RTX adhesins are long, multi-domain proteins present on the outer membrane of many Gram-negative bacteria. To expand the reach of the ligand-binding domains, RTX adhesins maintain a central extender region of multiple tandem repeats, which makes up most of the proteins’ large molecular weight. In this study, we analyzed extender regions from two additional RTX adhesins, including the long adhesion proteins from Marinobacter hydrocarbonoclasticus (MhLap) – an oil-eating marine bacterium – and Aeromonas hydrophila (AhLap) – an opportunistic pathogen of fish and mammals. However, all the tetra-tandemers have at least one calcium ion coordinated in the linker region between beta-sandwich domains whose role appears to be the rigidification of the extender region to help the adhesin extend its reach.

Calcium SAD phasing (Guo et al., 2019a, Guo et al., 2019b) was used to solve the tetra-tandemer structures to 2.0 Å (MhLap) and 1.75 Å resolution (AhLap). The repeats are rotated relative to each other around the long central axis, producing a handedness to the tetra-tandemers reminiscent of helices. Both the MhLap and AhLap structures show right-handed rotations, with pitches of approximately i + 3 and i + 2, respectively. Alternatively, the AhLap repeats possess a more involved connectivity, resulting in 50 Å-long beta sandwiches that are held together by one four-stranded and another five-stranded beta sheet. The AhLap tetra-tandemer coordinates many more calcium ions throughout its length than does MhLap, although the number of ions per repeat is inconsistent. Each inter-domain interface contains, at minimum, three highly coordinated Ca2+, labelled as calciums I, II, and III. Of the three, calcium I has the fewest coordinate bonds to protein-based ligands, with two positions in its six-ligand octahedral coordination sphere being taken up by water molecules. Both calciums II and III have pentagonal bipyramid coordination spheres, comprised of seven protein-based ligands each. The three Ca2+ are all coordinated by a combination of Asp, Asn, and Glu sidechains that are conserved in every repeat of the full-length adhesin (except the Glu in position 7, which is a comparable Gln for five repeats), as well as backbone carbonyl groups. Interestingly, several acidic residues (namely ligands 3, 6) use their bidentate sidechains to coordinate two separate calcium ions at the same time, making calciums I, II and III part of an interconnected coordination network. The AhLap structure was solved with two tetra-tandemers in the asymmetric unit, meaning that the structure holds eight repeat domains with six replicate interfaces between them. Of those six, four of them hold an additional calcium. In fact, the AhLap tetra-tandemer appears more rigid than the MhLap, with both angles remaining closer to the start angle over the entirety of the run.

>[2x]MASSHHHHHHSSGLVPRGSHMNDAAVITGSDTGAVTEDESTPLLTETGTLSVTDVDGADEAKFQAGNGTPSAGALGSLTITEGGAWTYNVDNSKVQYLGEGETKVETFTVASVDGTTHTVTITITGVNDAAVITGSDTGAVTEDESNPTLTETGTLSVTDVDGADEAKFLAGNGTPSAGALGSLTITEGGAWTYNVDNSKVQYLGEGETKVETFTVASVDGTTHTVTITITGVNDAAVISGSDTGAVTEDESTPLLTETGTLSVTDVDGADEAKFLAGNGVASNGALGSLTITEGGAWTYNVDNSKVQYLGEGETKVETFTVASVDGTTHTVTITITGVNDAAVISGSDTGAVTEDETNPLLTETGTLSVTDVDGADEAKFLAGNGTPSAGALGSLTITEGGAWTYNVDNSKVQYLGEGETKVETFTVASVDGTTHTVTITITGVNDGA>GSAKIPFYIMEEHNEAFFIWHYAVAEGWINKNQNTLLHVDEHSDLVVPILNSSLKSVNENIKRVHDFTYSELTIANFIYPALYQGVFSQVYWLRQKHDPKLNGQKQLNIYSHQGEGKRLILKSKVDFNNLFNPDCKSFTITPLNAQDDLSSEESKKLNKSVILDIDIDYFSCDNVSGEYLEVEITEEAYYDYINNLYNKLRICWGGNASVKYMDGKYYFCIIQPDKLVAENLKVSEDAIVERIDALIDFLKVNEIQPKLIDVCRSRLSGYTPNDQWEF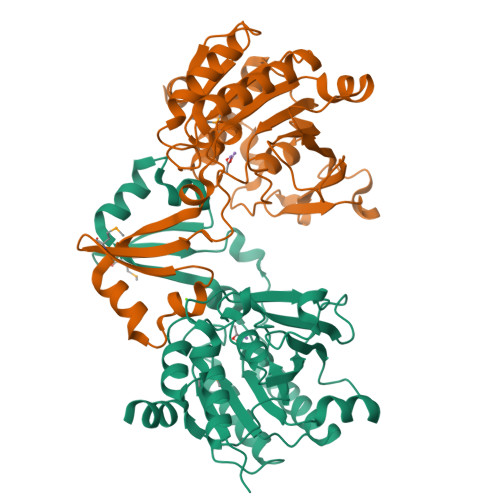IENTLVEKLSSIYEFEPIFVSELSKKVLVEV[4x]> MSEIGTGFPFDPHYVEVLGERMHYVDVGPRDGTPVLFLHGNPTSSYLWRNIIPHVAPSHRCIAPDLIGMGKSDKPDLDYFFDDHVRYLDAFIEAVGLEEVVLVIHDWGSALGFHWAKRNPERVKGIACMEFIRPIPTWDEWPEFARETFQAFRTADVGRELIIDQNAFIEGVLPKCVVRPLTEVEMDHYREPFLKPVDREPL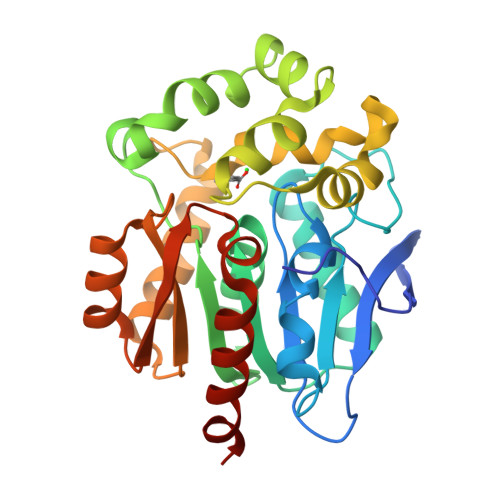WRFPNELPIAGEPANIVALVEAYMNWLHQSPVPKLLFWGTPGVLIPPAEAARLAESLPNCKTVDIGPGLHYLQEDNPDLIGSEIARWLPALHHHHHH>XGALEEIAQALEEIAKALKKIAWALKKIAQGX[6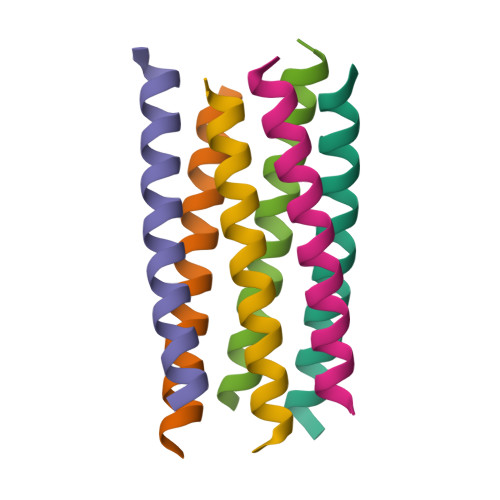x]> MAPLETIYDESLNKSADSIDDKKWSKLFPRIVSDPDRSSNFMTRAIYVAFSAVLRNRNILGQEYFTKNYITEKLKCMTLCFRNL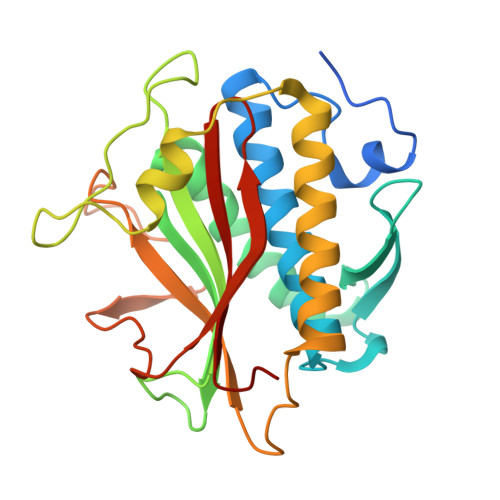RSNQIAQLLRNAGDATKDGFLKEVSLVITNNEGDLEAIEVFSMKFIYFENGGVVARLSTDKNGQEDPHFAKLAQLVYEGGDSVRDQMVTIVRSVQFLCTKVLEPLPEEFTANFRLEYTNDAPSNFRIDGFEDSSTFYTLPDDIQSATIGHLRPGCHAANMECWSMLMSD(2S)-2-azanyl-6-[(2-chlorophenyl)methoxycarbonylamino]hexanoic 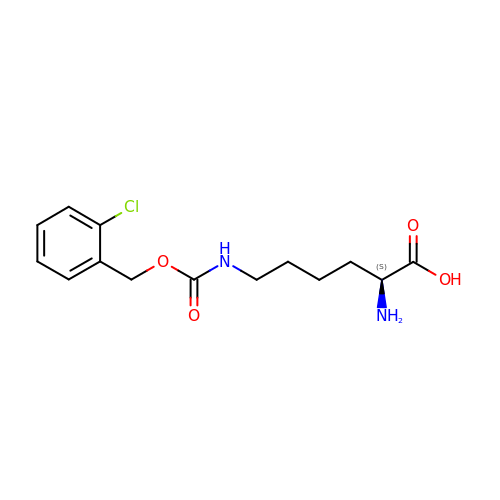acid | C14 H19 Cl N2 O4 | YCQVFPIEKSYHFI-LBPRGKRZSA-N>MALVVQKYGGSSLESAERIRNVAERIVATKKAGNDVVVVCSAMGDTTDELLELAAAVNPVPPAREMDMLLTAGERISNALVAMAIESLGAEAQSFTGSQAGVLTTERHGNARIVDVTPGRVREALDEGKICIVAGFQGVNKETRDVTTLGRGGSDTTAVALAAALNADVCEIYSDVDGVYTADPRIVPNAQKLEKLSFEEMLELAAVGSKILVLRSVEYARAFNVPLRVRSSYSNDPGTLIAGSMEDIPVEEAVLTGVATDKSEAKVTVLGISDKPGEAAKVFRALADAEINIDMVLQNVFSVEDGTTDITFTCPRSDGRRAMEILKKLQVQGNWTNVLYDDQVGKVSLVGAGMKSHPGVTAEFMEALRDVNVNIELISTSEIRISVLIREDDLDAAARALHEQFQLGGEDEAVVYAGTGR[8x];>MEEAVLTGVATDKSEAKVTVLGISDKPGEAAKVFRALADAEINIDMVLQNVFSVEDGTTDITFTCPRSDGRRAMEILKKLQVQGNWTNVLYDDQVGKVSLVGAGMKSHPGVTAEFMEALRDVNVNIELIST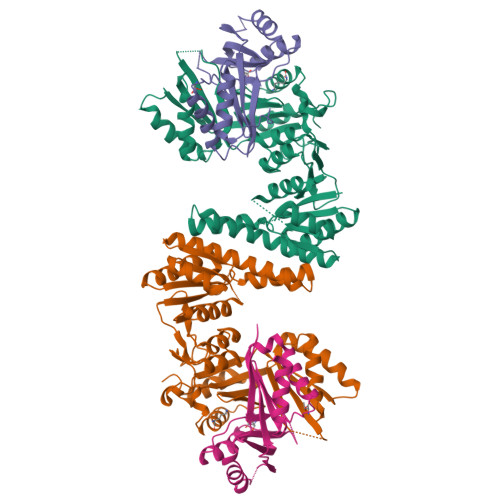SEIRISVLIREDDLDAAARALHEQFQLGGEDEAVVYAGTGRHHHHHH[8x]> GPSNITFYFPFGHVPTYGGDFVNLEHIRALNKHGFSAKVILMKNQIPIVIESFPKDIPVVFYKPGMELNAQDVFVLSEGVRIMYSGLA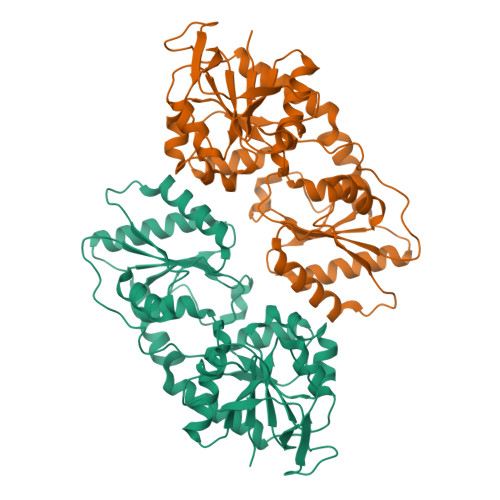QTQAFRVIVHNQNPFYTHTGMDSAHDINRYRITKIITPSHYTVKKLEEMGITKPMAVISPYIPEYFKPAEKSNEEIRITYSRRKREEESKILLFYLRSLYRGKKALHIRNLTNYKREEVAEEMSKAHIYASFAERESLGLMALEAMASGCHVVGFSGFTDFENQDVFNEENGDWVKEGEYKKFAEKLIEAIEQIENNTPSPKIENGLALVNSRFRQDRFEQEVVRVYQDILDNLPPLEGFNESDKVVLDFWHFD> MVKRTVATNGDASGAHRAKKMSKTHASHIINAQEDYKHMYLSVQPLDIFCWGTGSMCELGLGPLAKNKEVKRPRLNPFLPRDEAKIISFAVGGMHTLALDEESNVWSWGCNDVGALGRDTSNAKEQLKDMDADDSSDDEDGDLNELESTPAKIPRESFPPLAEGHKVVQLAATDNMSCALFSNGEVYAWGTFRCNEGILGFYQDKIKIQKTPWKVPTFSKYNIVQLAPGKDHILFLDEEGMVFAWGNGQQNQLGRKVMERFRLKTLDPRPFGLRHVKYIASGENHCFALTKDNKLVSWGLNQFGQCGVSEDVEDGALVTKPKRLALPDNVVIRSIAAGEHHSLILSQDGDLYSCGRLDMFEVGIPKDNLPEYTYKDVHGKARAVPLPTKLNNVPKFKSVAAGSHHSVAVAQNGIAYSWGFGETYAVGLGPFEDDTEVPTRIKNTATQDHNIILVGCGGQFSVSGGVKLSDEDAEKRADEMDD;> MDNGTDSSTSKFVPEYRRTNFKNKGRFSADELRRRRDTQQVELRKAKRDEALAKRRNFIPPTDGADSDEEDESSVSADQQFYSQLQQELPQMTQQLNSDDMQEQLSATVKFRQILSREHRPPIDVVIQAGVVPRLVEFMRENQPEMLQLEAAWALTNIASGTSAQTKVVVDADAVPLFIQLLYTGSVEVKEQAIWALGNVAGDSTDYRDYVLQCNAMEPILGLFNSNKPSLIRTATWTLSNLCRGKKPQPDWSVVSQALPTLAKLIYSMDTETLVDACWAISYLSDGPQEAIQAVIDVRIPKRLVELLS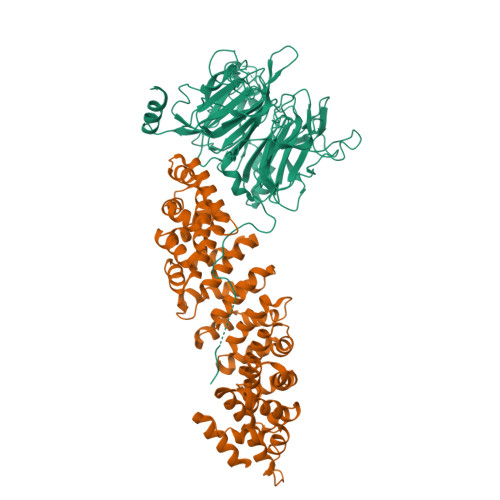HESTLVQTPALRAVGNIVTGNDLQTQVVINAGVLPALRLLLSSPKENIKKEACWTISNITAGNTEQIQAVIDANLIPPLVKLLEVAEYKTKKEACWAISNASSGGLQRPDIIRYLVSQGCIKPLCDLLEIADNRIIEVTLDALENILKMGEADKEARGLNINENADFIEKAGGMEKIFNCQQNENDKIYEKAYKIIETYFGEEEDAVDETMAPQNAGNTFGFGSNVNQQFNFN{(1R,2R,3S,4R)-4-[(5-{4-[(1S)-1-(6-bromopyridin-2-yl)-1-hydroxyethyl]thiophene-2-carbonyl}pyrimidin-4-yl)amino]-2,3-dihydroxycyclopentyl}methyl sulfamate | C22 H24 Br N5 O7 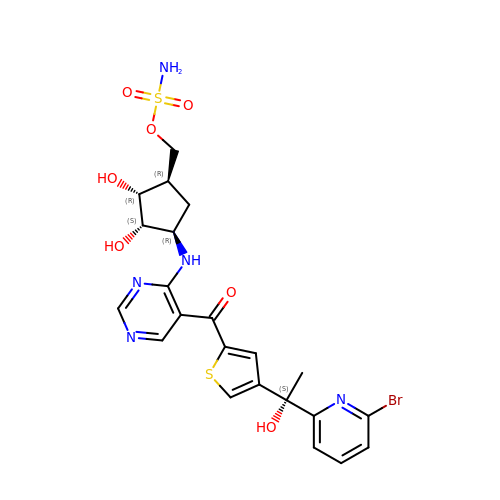S2 | IZYVMHSGDZFGFW-SULQKKJVSA-N> HHSRVSVAARDGSFTVSAQKNVEHGIIYIGKPSLRKQRFMQFSSLEHEGEYYMTPRDFLFSVMFEQMERKTSVKKLTKKDIEDTLSGIQTAGCGSTFFRDLGDKGLISYTEYLFLLTILTKPHSGFHVAFKMLDTDGNEMIEKREFFKLQKIISKQDDLMTVKTNETGYQEAIVKEPEINTTLQMRFFGKRGQRKLHYKEFRRFMENLQTEIQEMEFLQFSKG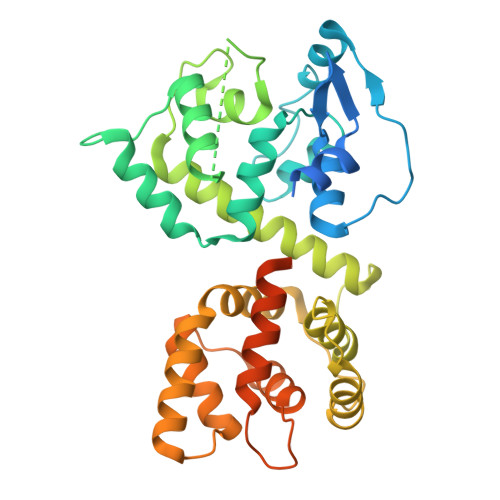LSFMRKEDFAEWLLFFTNTENKDIYWKNVREKLSAGESISLDEFKSFCHFTTHLEDFAIAMQMFSLAHRPVRLAEFKRAVKVATGQELSNNILDTVFKIFDLDGDECLSHEEFLGVLKNRMHRGLWVPQHQSIQEYWKCVKKESIKGVKEVWKQAGKGLF>[3x]SDLIPAPPLSKVPLQQNFQDNQFQGKWYVVGLAGNAILREDKDPQKMYATIYELKEDKSYNVTSVLFRKKKCDYWIRTFVPGSQPGEFTLGNIKSYPGLTSYLVRVVSTNYNQHAMVFFKKVSQNREYFKITLYGRTKELTSELKENFIRFSKSLGLPENHIVFPVPIDQCIDG

Siderocalin/Lipocalin 2/Neutrophil Gelatinase Associated Lipocalin/24p3 is an innate immune system protein with bacteriostatic activity, acting by tightly binding and sequestering diverse catecholate and mixed-type ferric siderophores from enteric bacteria and mycobacteria. Despite limited sequence similarity beyond minimal fold-defining motifs, lipocalins, including Scn (Coles et al., 1999, Goetz et al., 2000), display a common structural architecture: an eight-stranded antiparallel β-barrel enclosing a cup-shaped ligand binding site, or calyx. The calyx is strongly electropositive overall, due to the close arrangement of the side-chains of two lysines (K125, K134) and an arginine (R81), which complements the net negative charge of many ferric siderophores. Scn displays exceptional structural rigidity, manifested by its near-identical structure across multiple crystal structures, bound to a series of distinct ligands, tolerating multiple mutations.

P. aeruginosa produces two chemically-distinct siderophores, pyoverdine (PVD) and PCH, with relatively high or low affinities for iron, respectively. We had previously shown that Scn does not appreciably bind to PVD or PCH in qualitative binding assays, and does not arrest the growth of P. aeruginosa in vitro, suggesting that Scn does not efficiently sequester one or both siderophores. The quite large PVD structure would also not be expected to fit within the Scn calyx, nor would the structure of PCH-chelated iron be expected to fit within the key binding pocket, due to tight steric constraints around the iron center imposed by K125 and K134. A preliminary crystal structure of a Scn/PCH complex (3U03.pdb) was deposited in the Protein Databank (PDB,) by a structural genomics consortium. However, examination of this structure revealed a number of concerns. First, using the deposited diffraction data, it was readily apparent that the PCH ligand as modeled sat in negative electron density in difference Fourier syntheses. Second, this particular crystal form of Scn usually contains three molecules in the asymmetric unit, though only two had been modeled in the deposited structure. Using the deposited diffraction data, we re-refined the structure, successfully placing the third Scn molecule and improving refinement statistics: Rfree/Rwork values decreased from 0.303/0.269 (3U03.pdb) to 0.253/0.235. Calyx electron density features in the re-refined structure were inconsistent with bound Fe-PCH but were consistent with a bound sulfate ion comparable to those observed in apo-Scn structures crystallized from ammonium sulfate, and in the phenylurea complex. We concluded that Scn does not bind PCH, at least under these crystallization conditions, in concordance with prior results.>[2x]GQQPVNHLVKEIDMLLKEYLLSGDISEAEHCLKELEVPHFHHELVYEAIVMVLESTGESAFKMILDLLKSLWKSSTITIDQMKRGYERIYNEIPD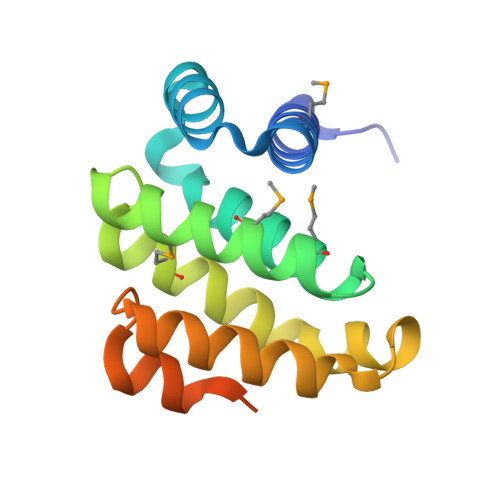INLDVPHSYSVLERFVEECFQAGIISKQLRDLCPSRGRKRFVSEGDGGRLKPESY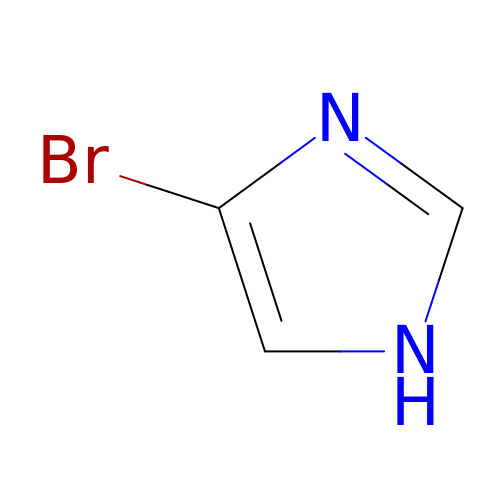4-bromo-1H-imidazole | C3 H3 Br N2 | FHZALEJIENDROK-UHFFFAOYSA-N>[2x]GEFNTIQQLMMILNSASDQPSENLISYFNNCTVNPKESILKRVKDIGYIFKEKFAKAVGQGCVEIGSQRYKLGVRLYYRVMESMLKSEEERLSIQN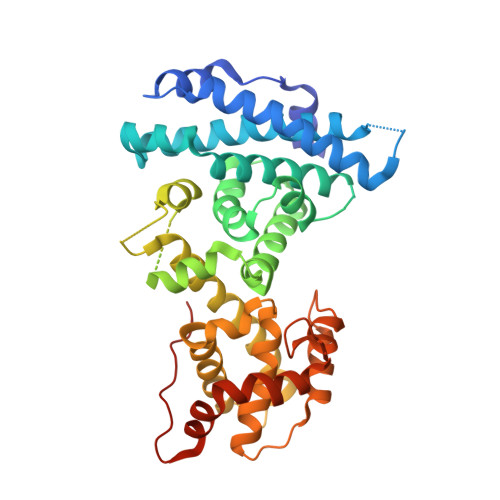FSKLLNDNIFHMSLLACALEVVMATYSRSTSQNLDSGTDLSFPWILNVLNLKAFDFYKVIESFIKAEGNLTREMIKHLERCEHRIMESLAWLSDSPLFDLIKQSKDREGPTDHLESACPLNLPLQNNHTAADMYLEPVRAPKKKSTSLSLFYKKVYRLAYLRLNTLCERLLSEHPELEHIIWTLFQHTLQNEYELMRDRHLDQIMMCSMYGICKVKNIDLKFKIIVTAYKDLPHAVQETFKRVLIKEEEYDYIIVFYNSVFMQRLKTNILQYASTRPPTLAPIPHIPRSPYKFP>MAPKRKASSTCKTPKRQCIPKPGCCPNVASVPKLLVKGGVEVLSVVTGEDSITQIELYLNPRMGVNSPDLPTTSNWYTYTYDLQPKGSSPDQPIKENLPAYSVARVSLPMLNEDITCDTLQMWEAISVKTEVVGISSLINVHYWDMKRVHDYGAGIPVSGVNYHMFAIGGEPLDLQGLVLDYQTQYPKTTNGGPITIETVLGRKMTPKNQGLDPQAKAKLDKDGNYPIEVWCPDPSKNENSRYYGSIQTGSQTPTVLQFSNTLTTVLLDENGVGPLCKGDGLFISCADIVGFLFKTSGKMALHGLPRYF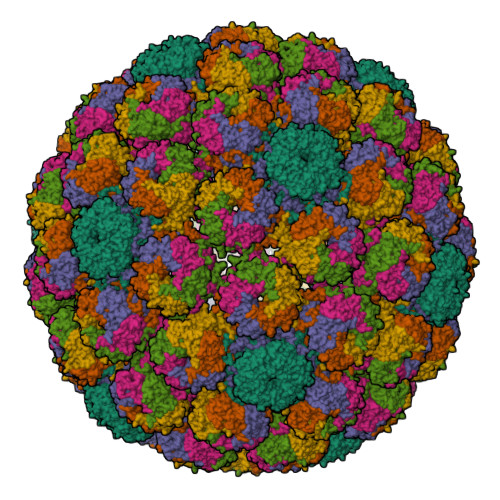NVTLRKRWVKNPYPVVNLINSLFSNLMPKVSGQPMEGKDNQVEEVRIYEGSEQLPGDPDIVRFLDKFGQEKTVYPKPSVAPAAVTFQSNQQDKGKAPLKGPQKASQKESQTQEL[6x]Spiroviolene synthase (SvS) from Streptomyces violens was first described by Rabe et al. and represents a bacterial class I diterpene cyclase that we were not able to produce in sufficient quantities for crystallization due to protein instability. Terpene cyclases such as SvS form a variety of complex multicyclic compounds with potent biological activities via carbocationic, electrophilic cyclization cascades of relatively simple substrates, either by metal-ion assisted release of an allylic pyrophosphate (class I mechanism) or by protonation of an oxirane/ene-functionality (class II mechanism). We previously reported a hypothetical ancestor of SvS—SvS-A2 26—which shares 77% sequence identity with the extant enzyme.

SvS-A2 forms a homodimer in solution, which was confirmed by size exclusion chromatography, consistent with the dimer found in the asymmetric unit of the crystal unit cell. Each monomer harbors one active site which points away from the dimer interface, resulting in an overall antiparallel arrangement. One of the two modeled loops comprises a conserved RY-dimer of bacterial terpene cyclases in the C-terminal end of helix K (312PRYLSL318), which adopts a helical structure in the GGPP-docked model. In SdS, a catalytic effector motif consisting of a phosphate sensor, a linker-residue, and an effector residue was described to mediate an induced-fit conformational rearrangement upon substrate binding, positioning the backbone carbonyl of the effector residue in closer proximity to the substrate. A functionally equivalent motif (Arg182, Ser185, and Ala186, shown in light green in Figure 1) is present in SvS-A2. Since this motif exhibits a similar orientation in the unliganded crystal structure as in the substrate-docked model (local Cα root-mean-square deviation (rmsd) of 0.22 Å over five residues) as well as substrate-bound SdS (Cα rmsd 0.30 Å over five residues), an equivalent induced fit rearrangement would likely occur to a lesser extent in SvS-A2. While the active site lining is virtually conserved between SvS-A2 and SvS-WT, the majority of ancestral mutations are hydrophilic and dispersed on the surface of SvS-A2. The generated homology models differ in the conformation of the modeled capping loop K. In SvS-WT-Hom1 (as well as in SvS-A2) this sequence adopts a helical fold and points to the surface of the enzyme, appearing to prevent full closure of the active site cleft (top row). Studying enzyme kinetics with individual substrates revealed that SvS-A2 exhibits well-defined cooperativity for spiroviolene production with a Hill-coefficient of 2.1 ± 0.4, whereas it was previously shown that SvS-WT could not be saturated with GGPP.

>MAMTVTEVDLPPIYCPLESAIHPRVHEVEKRAVEWIRRSGMCASEEERAWVIATHSADFFARFAPTAADEDRLLATSLWVYWGFAFDDARCDNGPLSTRPAQFNALAGRVQRALEAPSAEDNGDRFVPALQDIARRFRSFGTPTQVRRFVHAHRAWLSGVAWQIGNQARGHMPGLDDYLAMRLLSAGGEPTFAMLEIATGAEVPDREMHRPAVRALTEMAIMVAALDNDRHSLRKELSRGHTDQNIYSVLMHHRGMSLQEAVEEATKLRDRILLRFLELHDRVRPGAGAELSTYLQGLRHGIRGNAEWGLRVPRYLSLGRVPDPMEDAPLTWAESPSDSSPSPLPGAPSIAWWWDDALLGA[2x]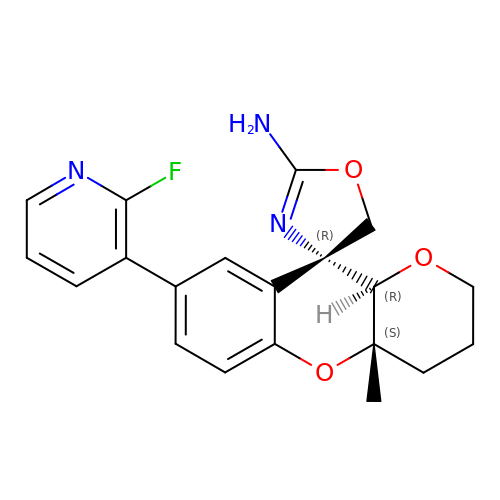(4R,4a'S,10a'R)-8'-(2-fluoropyridin-3-yl)-4a'-methyl-3',4',4a',10a'-tetrahydro-2'H-spiro[1,3-oxazole-4,10'-pyrano[3,2-b]chromen]-2-amine | C20 H20 F N3 O3 | DMNHLGOPJBTFQJ-IHPCNDPISA-N>MLPERVLEILREMKRERIKGASWLAKKGAEAFLTLAEELDESLLEDAIMELREEVVKVNPSMASLYNLARFIPVTNRRDILKSRALEFLRRMEEAKRELASIGAQLIDDGDVII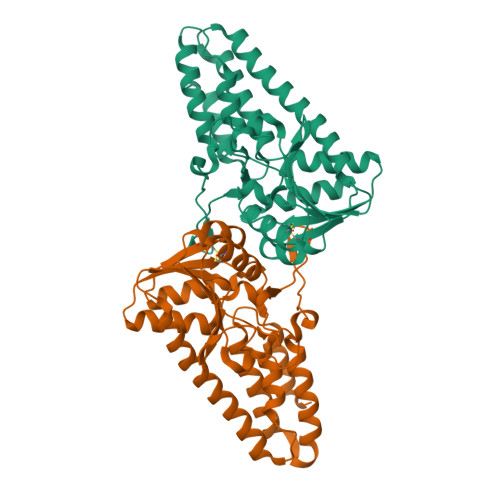THSFSSTVLEIIRTAKERKKRFKVILTESSPDYEGLHLARELEFSGIEFEVITDAQMGLFCREASIAIVGADMITKDGYVVNKAGTYLLALACHENAIPFYVAAETYKFHPTLKSGDVMLMERDLIRGNVRIRNVLFDVTPWKYVRGIITELGIVIPPRDIQ[2x]> MRTFFVGGNWKANPKTV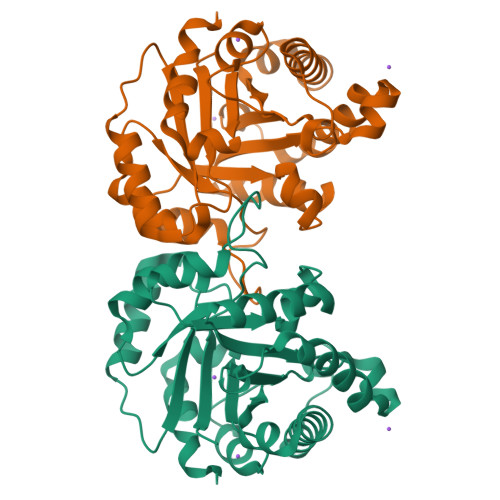EEAEKLIEMLNGAKVEGNVEVVVAAPFLFLPTLQQKLRKDWKVSAENVFTKPNGAFTGEVTVPMIKSFGIEWTILGHSERRDILKEDDEFLAAKAKFALENGMKIIYCCGEHLSEREAGKASEFVSAQIEKMIPAIPAGKWDDVVIAYEPIWAIGTGKVASTQDAQEMCKVIRDILAAKVGADIANKVRILYGGSVKPNNCNELAACPDVDGFLVGGASLEPGFINIVNSNVHSK> DCPSGWSSYEGHCYKPFKLYKTWDDAERFCTEQAKGGHLVSIESAGEADFVAQLVTENIQNTK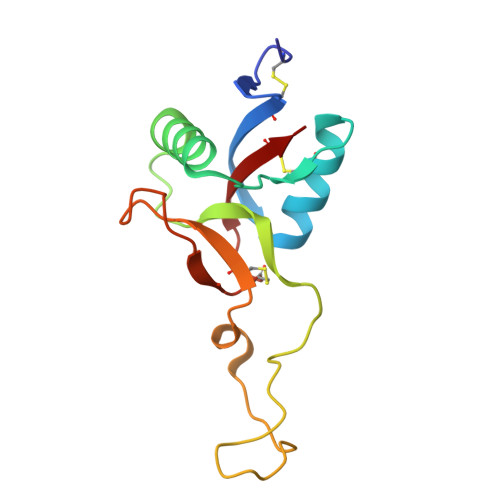SYVWIGLRVQGKEKQCSSEWSDGSSVSYENWIEAESKTCLGLEKETGFRKWVNIYCGQQNPFVCEA>MGNYLEDCATVDVQARPTAYALAISSLGEFNSLTGGTSTDPVAEGNDYYYRFEIRAWEGSSGPQTNVTLNVTRTLGNSTFAGSGTKGVDFEVELDPDGPFGPASYAPVLSADVQVLAWGPTGVQLRYLPSLAPGATLRFSLRANA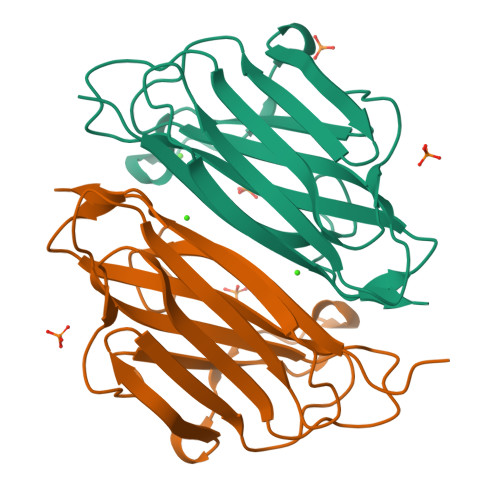VNGTNTTVQADATSTEAPGPYTVFETTTIIP[2x]5-bromo-2'-deoxycytidine | C9 H12 Br N3 O4 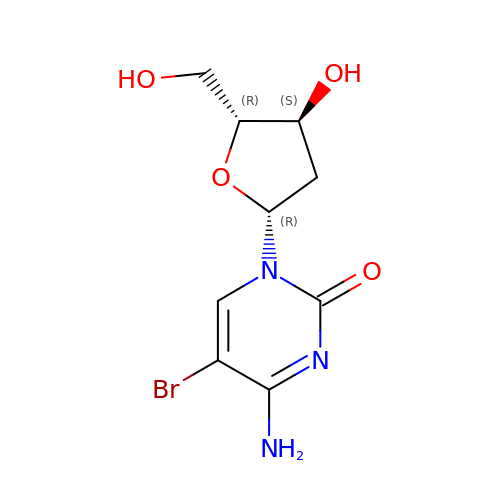| KISUPFXQEHWGAR-RRKCRQDMSA-N>[4x]MLKAWHLPVAPFIKEQQERLMITLWLSGDDLPPRVTLRAEEDNEELSLPMHRLRQAPHPGVVAWRGEINLVNGQPRRRYSFKLLWADRQLWFTPQEFNRFPPARLEQFAVDLPDSGPQWVADQVFYQIFPDRFARSQSHDIVRKAWDEPLTAEAGGSTFYGGDLDGISEKLPYLKQLGVTALYLNPVFVAPSVHKYDTEDYRRVDPQFGGDAALLRLRHNTQKEGMRLILDGVFNHSGDSHYRSSTLIDEIYGGEDSVVRHWLKAPWSMDG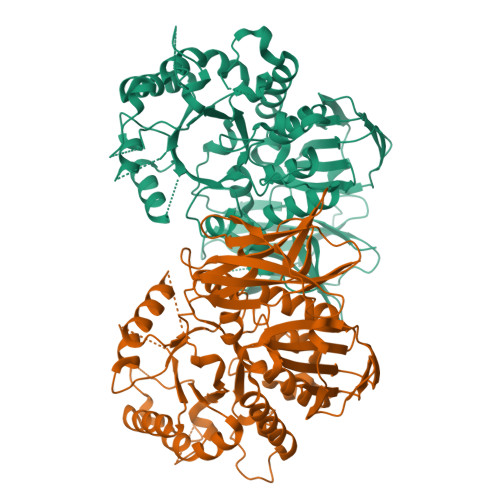WRLDVVHMLGEGGGARNNLRHIAGITQAAKLERPDAFVFGEHFGDARQWLQADVEDSAMNYRGFTFPLWGFLANTDISYDPQKIDAQTCMAWMDNYRAGLSHQQQLRMFNQLDSHATARFKSLLGKDVARLPLAVVWLFSWPGVPCIYYGDEVGVDGNNDPFCRKPFPWDPALQDGDLLDLYKRMSKLRKAHQALRYGGCQVIYAEDNVVVFVRVYKQQRVLVAINRGEACEVVIEDSPLLDVNGWQLKEGAGALHDGVLTLPAISASVWFSR>QANLMRLKSDLFNRSPMYPGPTKDDPLTVTLGFTLQDIVKVDSSTNEVDLVYCEQQRWKLNSLMWDPNEYGNITDFRTSAADIWTPDITAYSSTRPVQVLSPQIAVVTHDGSVMFIPAQRLSFMCDPTGVDSEEGVTCAVKFGSWVYSGFEIDLKTDTDQVDLSSYYASSKYEILSATQTRQVQHYSCCPEPYIDVNLVVKFRE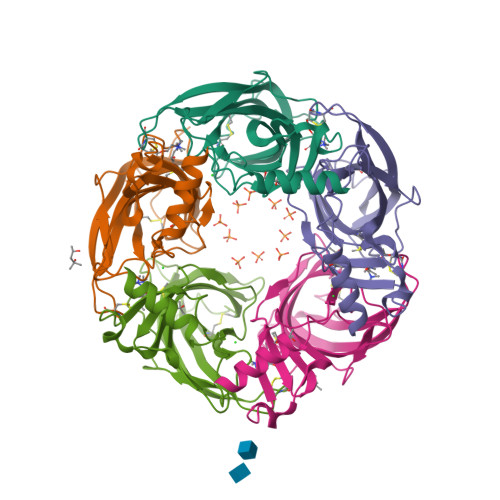RRAGNGFFRNLFD[5x]Acyl-CoA:diacylglycerol acyltransferase 1 (DGAT1) is one of two enzymes known to catalyze TG synthesis in humans. It esterifies diacylglycerol (DAG) with acyl-CoA to generate TGs at the endoplasmic reticulum (ER). DGAT1 belongs to the family of membrane-bound O-acyltransferases (MBOAT), with members in all kingdoms of life. Each enzyme has a catalytic center with evolutionarily conserved histidine and asparagine (aspartate for HHAT) residues that are embedded deeply within the ER membrane.

To ascertain how T863 inhibits DGAT1, we determined the cryo-EM structure of DGAT1 bound to this compound when reconstituted in amphipol PMAL-C8. The resulting DGAT1 cryo-EM dimer map resolved overall at ~3.2 Å resolution and was very similar to the structure of apo DGAT1 (0.73 Å RMSD of 406 aligned residues). The structure contains an additional density corresponding to one T863 molecule bound to each DGAT1 protomer. T863 resided at the end of the cytosol-facing acyl-CoA-binding tunnel of DGAT133. The positioning of T863 in acyl-CoA binding tunnel is consistent with previous results showing that the drug competes with the acyl-CoA substrate for enzyme binding. T863 interacts with DGAT1 through both hydrophobic and polar interactions. For the bulky region of T863 that inserts into the fatty acid binding tunnel, the oxygen atom connecting C14 and C15 and the tertiary amine linking the C13 and C14 position form hydrogen bonds with the evolutionarily conserved residue Ser411. In addition, a primary amine at the C12 position forms hydrogen bonds with the main chain carbonyl groups of Trp374 and Trp377. Furthermore, the bulky region (7,7-dimethyl-7H-pyrimido(4,5-b)[1,4]oxazin-4-amine) that links to the cyclohexylbenzene moiety interacts with the catalytic residues His415 and Asn378 through hydrophobic interactions. While the overall structure of DGAT1 appears unaltered by T863 binding, a few residues at the drug-binding pocket, including Phe408 and Asn465 had subtle conformation changes, orienting them toward the T863 molecule.

>MGDRGSSRRRRTGSRPSSHGGGGPAAAEEEVRDAAAGPDVGAAGDAPAPAPNKDGDAGVGSGHWELRCHRLQDSLFSSDSGFSNYRGILNWCVVMLILSNARLFLENLIKYGILVDPIQVVSLFLKDPYSWPAPCLVIAANVFAVAAFQVEKRLAVGALTEQAGLLLHVANLATILCFPAAVVLLVESITPVGSLLALMAHTILFLKLFSYRDVNSWCRRARAKAASAGKKASSAAAPHTVSYPDNLTYRDLYYFLFAPTLCYELNFPRSPRIRKRFLLRRILEMLFFTQLQVGLIQQWMVPTIQNSMKPFKDMDYSRIIERLLKLAVPNHLIWLIFFYWLFHSCLNAVAELMQFGDREFYRDWWNSESVTYFWQNWNIPVHKWCIRHFYKPMLRRGSSKWMARTGVFLASAFFHEYLVSVPLRMFRLWAFTGMMAQIPLAWFVGRFFQGNYGNAAVWLSLIIGQPIAVLMYVHDYYVLNYEAPAAEA[2x]> GMQEHYQPAAIEPAAQKKWDDARISNVSEDASKPKYYCLSMFPYPSGKLHMGHVRNYTIGDVLSRFKLLNGFNVMQPMGWDAFGMPAENAAMKNNVAPAAWTYDNIEYMKTQLKSLGFAVDWEREVATCKPEYYRWEQWLFTKLFEKGIVYRKNGTVNWDPVDQTVLANEQVIDGRGWRSGALIEKREIPMYYFKITDYAEELLNDLDKLEHWPEQVKTMQRNWIGKSRGMTVRFAVSDDSKQGLEGDYAKFLQVYTTRPDTLMGATYVAVAAEHPLATAAAADKPELQAFIAECKAGSVAEADMATMEKKGVPTGRYVVNPLNGDKLEVWIANYVLWGYGDGAVMAVPAHDERDFEFAAKYNLPKKQVIAVGDNAFDANRWQEWYGDKENGVLVNSGDLDGLDFQTAFDAVAAKLQSQGAGE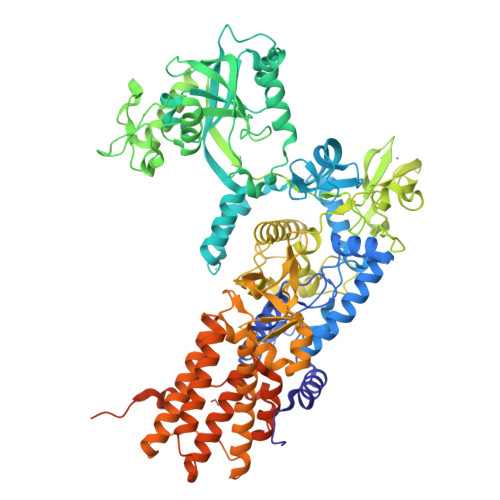PKTQYRLRDWGISRQRYWGCPIPIVHCEKCGNVPVPADQLPVVLPENVVPDGMGSPLAKMPEFYETSCPCCGGAAKRETDTMDTFIESSWYFFRYMSPKFSDGMVSAESAKYWGAVDQYIGGIEHAILHLLYARFFTKLMRDEGLVNVDEPFERLLTQGMVVCETYYRENDKGGKDWINPADVELTFDDKGRPVSAVLKADGLPVVISGTEKMSKSKNNGVDPQELINAYGADTARLFMMFAAPPEQSLEWSDSGVEGAHRFLRRLWRTVYEYLKQGGAVKAFAGNQDGLSKELKDLRHKLHSTTAKVSDDYGRRQQFNTAIAAVMELLNQYDKTDTGSEQGRAVAQEVLEAAVRLLWPIVPHICETLWSELNGAKLWEAGWPTVDEAALVKSEIEVMVQVNGKLRGKITVAADASKADLEAAALANEGAVKFMEGKPAKKIIVVPGRLVNIVV>MAPKAVLVGLPGSGKSTIGRRLAKALGVGLLDTDVAIEQRTGRSIADIFATDGEQEFRRIEEDVVRAALADHDGVLSLGGGAVTSPGVRAALAGHTVVYLEISAAEGVRRTGGNTVRPLLAGPDRAEKYRALMAKRAPLYRRVATMRVDTNRRN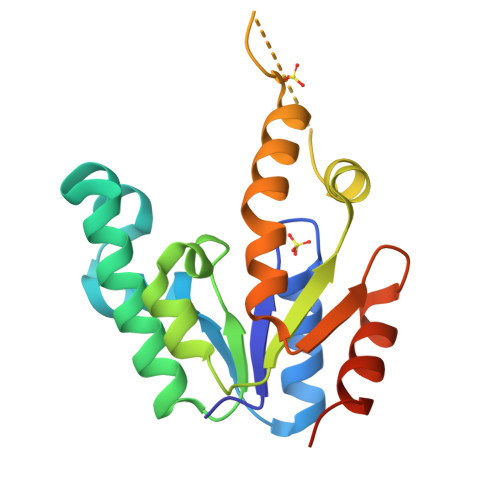PGAVVRHILSRLQVPSPSEAAT[2x]>[2x]DYKDDDDKAAAQSLEFNSPADNYTVCEGDNATLSCFIDEHVTRVAWLNRSNILYAGNDRWTSDPRVRLLINTPEEFSILITEVGLGDEGLYTCSFQTRHQPYTTQVYLIVHVPARIVNISSPVTVNEGGNVNLLCLAVGRPEPTVTWRQLRDGFTSEGEILEISDIQRGQAGEYECVTHNGVNSAPDSRRVLVTVNYPPTITDVTSARTALGR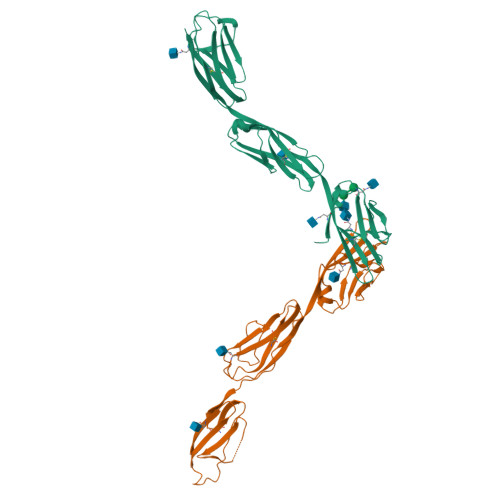AALLRCEAMAVPPADFQWYKDDRLLSSGTAEGLKVQTERTRSMLLFANVSARHYGNYTCRAANRLGASSASMRLLRPGSLENSALEVLFQ;>DYKDDDDKAAAVDFPWAAVDNMMVRKGDTAVLRCYLEDGASKGAWLNRSSIIFAGGDKWSVDPRVSISTLNKRDYSLQIQNVDVTDDGPYTCSVQTQHTPRTMQVHLTVQVPPKIYDISNDMTVNEGTNVTLTCLATGKPEPSISWRHISPSAKPFENGQYLDIYGITRDQAGEYECSAENDVSFPDVRKVKVVVNFAPTIQEIKSGTVTPGRSGLIRCEGAGVPPPAFEWYKGEKKLFNGQQGIIIQNFSTRSILTVTNVTQEHFGNYTCVAANKLGTTNASLPLNPPSTAQYGITGLEVLFQ[2x]>[2x]MVYYPKKYELYKADEVPTEVVETDILIIGGGFSGCGAAYEAAYWAKLGGLKVTLVEKAAVERSGAVAQGLSAINT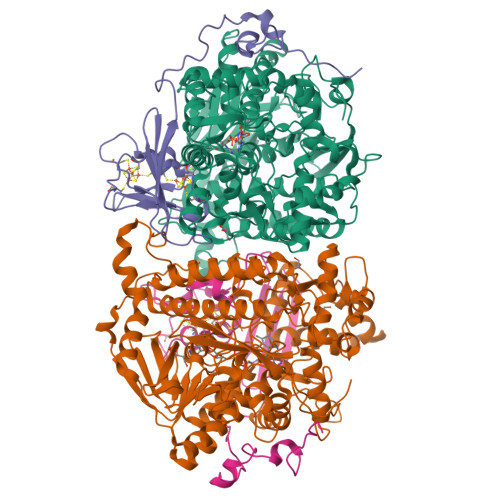YIDLTGRSERQNTLEDYVRYVTLDMMGLAREDLVADYARHVDGTVHLFEKWGLPIWKTPDGKYVREGQWQIMIHGESYKPIIAEAAKMAVGEENIYERVFIFELLKDNNDPNAVAGAVGFSVREPKFYVFKAKAVILATGGATLLFRPRSTGEAAGRTWYAIFDTGSGYYMGLKAGAMLTQFEHRFIPFRFKDGYGPVGAWFLFFKCKAKNAYGEEYIKTRAAELEKYKPYGAAQPIPTPLRNHQVMLEIMDGNQPIYMHTEEALAELAGGDKKKLKHIYEEAFEDFLDMTVSQALLWACQNIDPQEQPSEAAPAEPYIMGSHSGEAGFWVCGPEDLMPEEYAKLFPLKYNRMTTVKGLFAIGDCAGANPHKFSSGSFTEGRIAAKAAVRFILEQKPNPEIDDAVVEELKKKAYAPMERFMQYKDLSTADDVNPEYILPWQGLVRLQKIMDEYAAGIATIYKTNEKMLQRALELLAFLKEDLEKLAARDLHELMRAWELVHRVWTAEAHVRHMLFRKETRWPGYYYRTDYPELNDEEWKCFVCSKYDAEKDEWTFEKVPYVQVIEWSF;>MPSFVNPEKCDGCKALERTACEYICPNDLMTLDKEKMKAYNREPDMCWECYSCVKMCPQGAIDVRGYVDYSPLGGACVPMRGTSDIMWTVKYRNGKVLRFKFAIRTTPWGSIQPFEGFPEPTEEALKSELLAGEPEIIGTSEFPQVKKKA[2x]>[2x]GASTATVGRWMGPAEYQQMLDTGTVVQSSTGTTHVAYPADIDAFGKQAKNG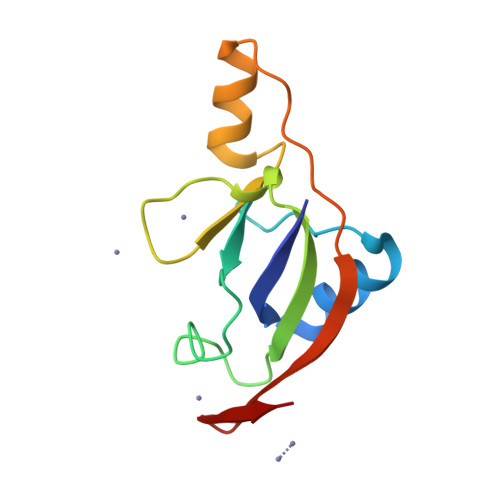AMYVEFDVPEKSLVPTNEGWAKIVGPDSIEGRLAKRKGLPVPEMPTAENITVRGEKINGEVEAKC> RAPDSVDYRKKGYVTPVKNQGQCGSCWAFSSVGALEGQLKKKTGKLLNLSPQNLVDCVSENDGCGGGYMTNAFQYVQKNRGIDSEDAYPYVGQEESCMYNPTGKAAKCRGYREIPEGNEKALKRAVARVGPVSVAIDASLTSFQFYSKGVYYDESCNSDNLNHAVLAVGYGIQKGNKHWIIKNSWGENWGNKGYILMARNKNNACGIANLASFPKM;> LYPEEILDTHWELWKKTHRKQYNNKVDEISRRLIWEKNLKYISIHNLEASLGVHTYELAMN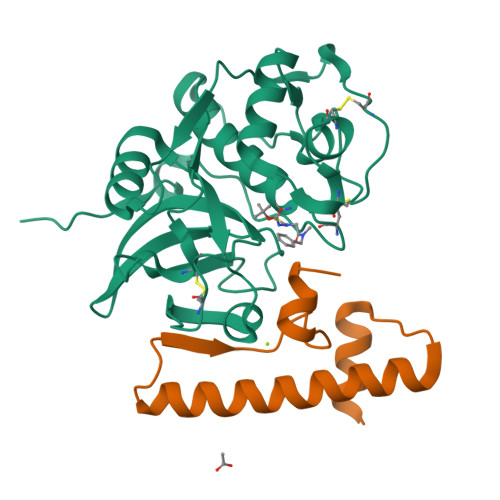HLGDMTSEEVVQK>DYGRADNENRVGQVTGLAWTEVGGDLLTIETACVPGKGKLTYTGSLGEVMQESIQAALTVVRARAEKLGINPDFYEKRDIHVHVPEGATPKDGPAAGIAMCTALVSCLTGNPVRADVAMTGEITLRGQVLPIGGLKEK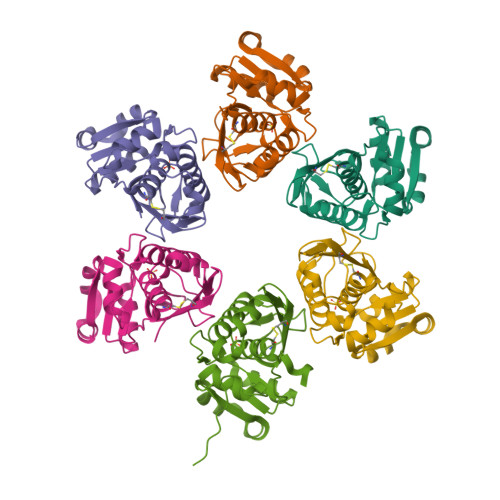LLAAHRGGIKTVLIPFENKRDLEEIPDNVIADLDIHPVKRIEEVLTLALQNEPSGMQVVTAK[6x]> PISPIETVPVKLKPGMDGPKVKQWPLTEEKIKALVEICTEMEKEGKISKIGPENPYNTPVFAIKKKDSTKWRKLVDFRELNKRTQDFWEVQLGIPHPAGLKKNKSVTVLDVGDAYFSVPLDEDFRKYTAFTIPSINNETPGIRYQYNVLPQGWKGSPAIFQSSMTKILEPFKKQNPDIVIYQYMDDLYVGSDLEIGQHRTKIEELRQHLLRWGLTTPDKKHQKEPPFLWMGYELHPDKWTVQPIVLPEKDSWTVNDIQKLVGKLNWASQIYPGIKVRQLSKLLRGTKALTEVIPLTEEAELELAENREILKEPVHGVYYDPSKDLIAEIQ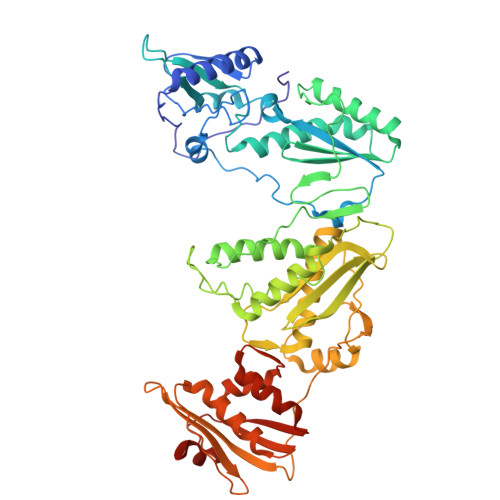KQGQGQWTYQIYQEPFKNLKTGKYARMRGAHTNDVKQLTEAVQKITTESIVIWGKTPKFKLPIQKETWETWWTEYWQATWIPEWEFVNTPPLVKLWYQLEKEPIVGAETFYVDGAANRETKLGKAGYVTNKGRQKVVPLTNTTNQKTELQAIYLALQDSGLEVNIVTDSQYALGIIQAQPDKSESELVNQIIEQLIKKEKVYLAWVPAHKGIGGNEQVDKLVSAGIRKIL> SMQAKGEAAMRDLIAELHAMQSPYTVQRFISSGSYGAVCAGVDSEGIPVAIKRVFNTVSDGRTVNILSDSFLCKRVLREIRLLNHFHHPNILGLRDIFVHFEEPAMHKLYLVTELMRTDLAQVIHDQRIVISPQHIQYFMYHILLGLHVLHEAGVVHRDLHPGNILLADNNDITICDFNLAREDTADANKTHYVTHRWYRAPELVMQFKGFTKLVDMWSAGCVMAEMFNRKALFRGSTFYNQLNKIVEVVGTPKIEDVVMFSSPSARDYLR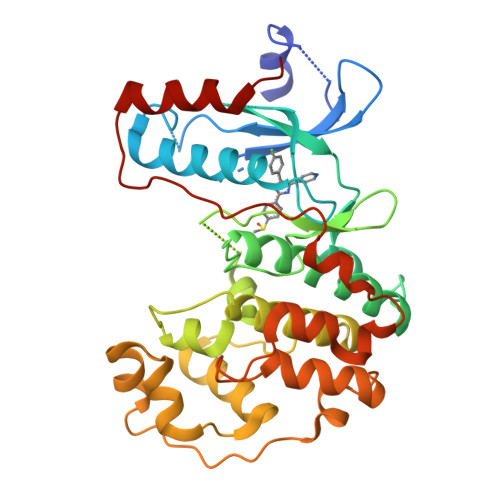NSLSNVPARAWTAVVPTADPVALDLIAKMLEFNPQRRISTEQALRHPYFESLFDPLDLTEGLSERFHFDESVTDVYDMHKIFTAEVERFND> MAFARGGLAQTASQTTSSPVRVGLSVDASALGHTIPPDYTGLSYEQAQMANPNYFSGANTQLAGFLRTLGRQGVLRI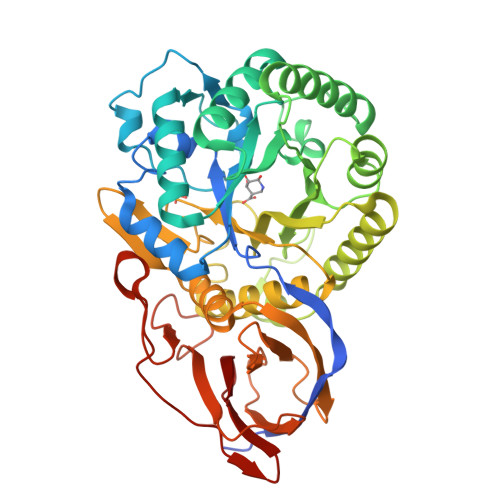GGNTSEYTFWNRHAKPTAADEHLAAGPDKGHHAAAREVITPEAVNNLSEFLDKTGWKLIYGLNLGKGTPENAADEAAYVMETIGADRLLAFQLGNEPDLFYRNGIRPASYDFAAYAGDWQRFFTAIRKRVPNAPFAGPDTAYNTKWLVPFADKFKHDVKFISSHYYAEGPPTDPSMTIERLMKPNPRLLGETAGLKQVEADTGLPFRLTETNSCYQGGKQGVSDTFAAALWAGDLMYQQAAAGSTGINFHGGGYGWYTPVAGTPEDGFIARPEYYGMLLFAQAGAGQLLGAKLTDNSAAPLLTAYALRGTDGRTRIALFNKNLDADVEVAISGVASPSGTVLRLEAPRADDTTDVTFGGAPVGASGSWSPLVQEYVPGHSGQFVLHMRKASGALLEFA>MELIRIAMKKDLENDNSLMNKWATVAGLKNPNPLYDFLNHDGKTFNEFSSIVNIVKSQYPDREYELMKDYCLNLDVKTKAARSALEYADANMFF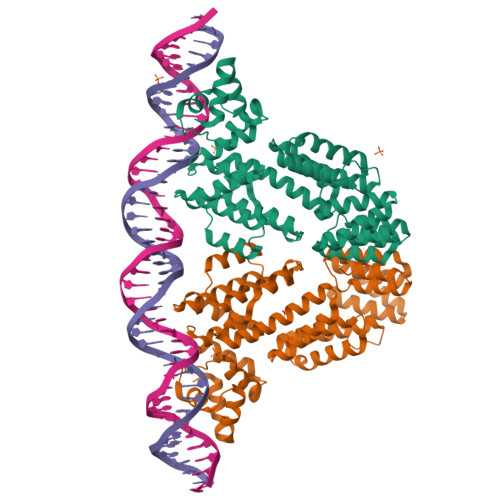EIEDVLIDSMISCSNMKSKEYGKVYKIHRELSNSVITEFEAVKRLGKLNIKTPEMNSFSRLLLLYHYLSTGNFSPMAQLIKQIDLSEISENMYIRNTYQTRVHVLMSNIKLNENSLEECREYSKKALESTNILRFQVFSYLTIGNSLLFSNYELAQENFLKGLSISVQNENYNMIFQQALCFLNNVWRKENKWINFESDSIMDLQEQAHCFINFNENSKAKEVLDKLDLLVHNDNELAMHYYLKGRLEQNKACFYSSIEYFKKSNDKFLIRLPLLELQKMGENQKLLELLLL[2x]>MSLKLIGMLDSPYVRRVAISLKSLGLPFEHHSLSVFSTFEQFKAINPVVKAPTLVCEGGEVLMDSSLIIDYLETLAGPQRSLMPTALPQRLRELRLVGLALAACEKSVQIVYERNLRPAEKQHGPWLERVGGQLQAAYGELEQELQKQPLPRDGSLGQAGISLAVAWSFSQMMVADQFNPGQFPAVRGFAEYAEQLPVFLATPATEGHHHHHH[4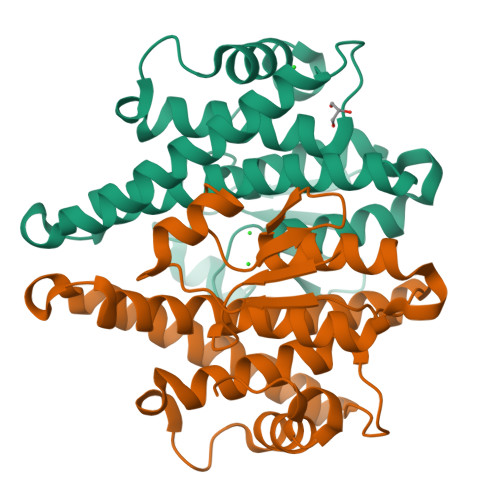x]Plexins are a large group of type I transmembrane proteins that serve as the major receptors for semaphorins. The plexin cytoplasmic region contains a juxtamembrane segment, a RhoGTPase binding domain (RBD) and a GTPase activating protein (GAP) domain. Instead it is active specifically to the Ras homolog Rap, and this RapGAP activity is critical for plexin signaling. Semaphorin binding to the plexin extracellular region induces formation of the active dimer of the cytoplasmic region, which triggers its GAP activity to inactivate Rap through the non-canonical catalytic mechanism for signal transduction.

To stabilize the interaction, we covalently linked plexinscyto and Rap1B in vitro by using a protein ligation system based on the transpeptidase activity of sortase from Staphylococcus aureus (see details in ‘Materials and methods’). We therefore used the γ-phosphate analog aluminum fluoride (AlFx, x = 3 or 4) to induce formation of the transition state complex between Rap(GDP) and plexin. We crystallized this complex with AlFx and determined the structure to 3.3 Å resolution. The asymmetric unit of the PlexinC1cyto/Rap1B complex structure contains four protomers of the complex, which are virtually identical to one another. The four PlexinC1 molecules form two pairs of dimers, consistent with the dimerization observed in solution. The GAP domain in PlexinC1 and Switches I (residues 30–38) and II (residues 59–67) in Rap constitute the majority of the binding interface, whereas the RBD in plexin is not involved and its role in GAP regulation remains unclear. The presumed arginine finger (Arg711) in PlexinC1 superimposes well with the arginine finger (Arg789) in p120GAP, playing the same role in catalysis by interacting with the AlFx and GDP in the active site. Switch II of Rap in the complex structure adopts an unprecedented conformation that is markedly different from both the p120GAP/Ras and the RapGAP/Rap complexes. Residues 60–63 in Switch II form a tight hairpin-like turn, which brings Gln63 close to AlF3 (therefore named the Gln63-in conformation). The Gln63-in conformation of Switch II is stabilized by numerous specific interactions between PlexinC1 and Rap.

>GGSSQKQMSKKMNDQLELMESNIRRDIRQGFVDLQTEKSDLIDNVGAIPFLDYKHFASRIFFPEAGTLTAVMIRDIGEDSEQTTVDEKCLAFAELIRDKQFLSCFVHALEEQKNFSIKDKCTVASLLTLALHGDLLYLTEIMEDLLQSLMDQSSNANPKLLLRRTESIVEKLLTNWMSICLYGFLRESVGQPLFLLVSALTQQISKGPVDSVTEKALYTLSEDWLLCQAQDFEPLKLKVVFAVGTGEEISESLEVIALTCDTIQQVKEKILQTFQRKFGFRYTQQIRDIEIEYEKEGKFVMLQEVDDTSEIRGHVTMLNTLKHYQVGDGACIKVITPKIHAPLKTQNSVKDDKNFSIKYFHLVDPDIDTDLSNHPEKKALKIKEMYLIKLLSTKVAVHSFVENLFKSIWGLPNNKAPLAVKYFFDFLDEQAERKKITDPDVLHIWKTNSLPLRFWVNILKNPDFVFSDMEKSPHLDGCLSVIAQAFMDSFSLTDTHLDKHSPTNKLLYGKDIPQYKQEVKSYYKLVKDQTSISSQELKTFLQEESKKHQNEFNESAALRELYKYMQRYFTEIFQKLEQTDAPSNLKENMHRVKELFDNM[4x];>[4x]GPHMREYKLVVLGSGGVGKSALTVQFVQGIFVEKYDPTIEDSYRKQVEVDAQQCMLEILDTAGTEQFTAMRDLYMKNGQGFALVYSITAQSTFNDLQDLREQILRVKDTDDVPMILVGNKCDLEDERVVGKEQGQNLARQWNNCAFLESSAKSKINVNEIFYDLVRQINSGGSGSGSSGGSGSGGGSGSGSSGLPETGG>[2x]MEIPVIEPLFTKVTEDIPGAAGPVFDKNGDFYIVAPYVEVNGKPAGEILRIDLKTGKKTVICKPEVNGYGGIPAGCQCDRDANQLFVADMRLGLLVVQTDGTFEEIAKKDSEGRRMQGCAYCAFDYEGNL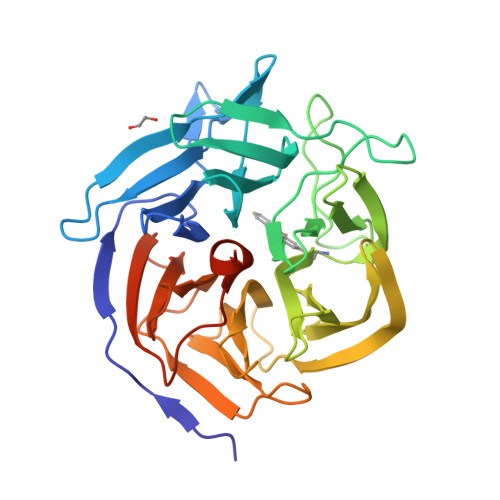WITAPAGEVAPADFTISLQEKFGSIYCFTTDGQMIQVDTAFQXPAGIAVRHMNDGRPYQLIVAEQPTKKLWSYDIKGPAKIENKKVWGHIPGTHKGGAAGMDFDEDNNLLVANWGSSHIEVFGPDGGQPKMRIRCPFEKPSALHFKPQTKTIFVTEHENNAVWKFEWQRNGKKQYCETLKFGIFGSLEWSHPQFEK> VFEVPKQNGKYETGQLFLHSIFGYRGVVLFPWQARLYDRDVASAAPEKAENPAGHGSKEVKGKTHTYYQVLIDARDCPHISQRSQTEAVTFLANHDDSRAL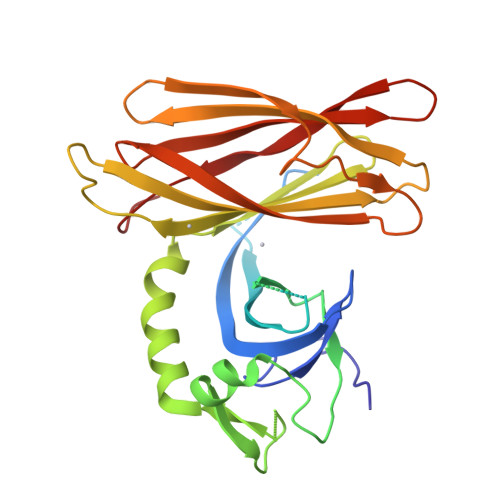YAIPGLDYVSHEDILPYTSTDQVPIQHELFERFLLYDQTKAPPFVARETLRAWQEKNHPWLELSDVHRETTENIRVTVIPFYMGMREAQNSHVYWWRYCIRLENLDSDVVQLRERHWRIFSLSGTLETVRGRGVVGREPVLSKEQPAFQYSSHVSLQASSGHMWGTFRFERPDGSHFDVRIPPFSLESNKDE> MATGTRYAGKVVVVTGGGRGIGAGIVRAFVNSGARVVICDKDESGGRALEQELPGAVFILCDVTQEDDVKTLVSETIRRFGRLDCVVNNAGHHPPPQRPEETSAQGFRQLLELNLLGTYTLTKLALPYLRKSQGNVINISSLVGAIGQAQAVPYVATKGAVTAMTKALALDE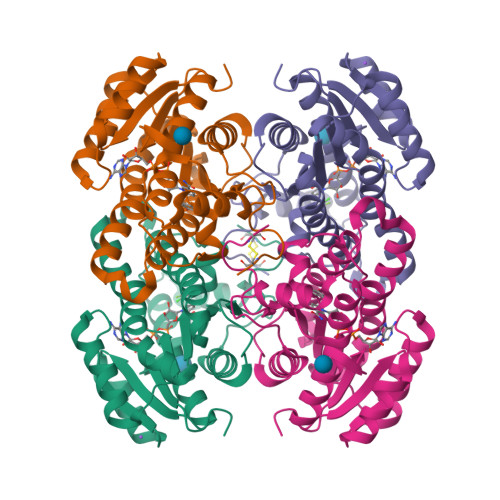SPYGVRVNCISPGNIWTPLWEELAALMPDPRASIREGMLAQPLGRMGQPAEVGAAAVFLASEANFCTGIELLVTGGAELGYGCKASRSTPVDAPDIPS>[2x]NQPVNQPILAAAQSLHQEATQWSSKGNDIIAAAKRMALLMAEMSRLVRGGSGTKRALIQC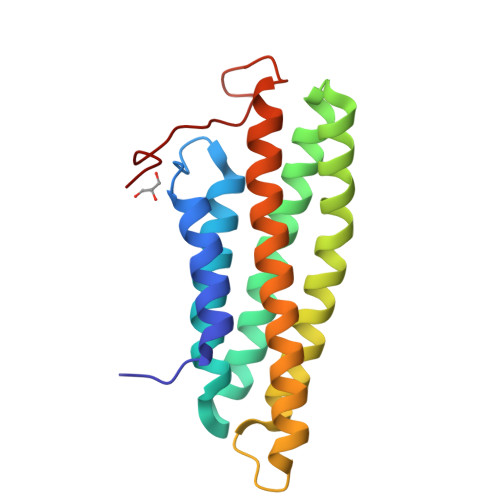AKDIAKASDEVTRLAKEVAKQCTDKRIRTNLLQVCERIPTISTQLKILSTVKATMLGRTNISDEESEQATEMLVHNAQNLMQSVKETVQEAEAASIKIRTDAGFTLRWVQKTPWYQ> EYIKLKVIGQDSSEIHFKVKMTTHLKKLKESYCQRQGVPMNSLRFLFEGQRIADNHTPKELGMEEEDVIEVYQE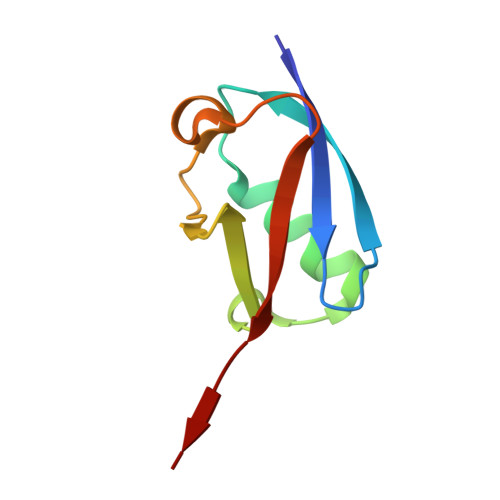QTGG TRANS-4-AMINOMETHYLCYCLOHEXANE-1-CARBOXYLIC ACID | C8 H15 N 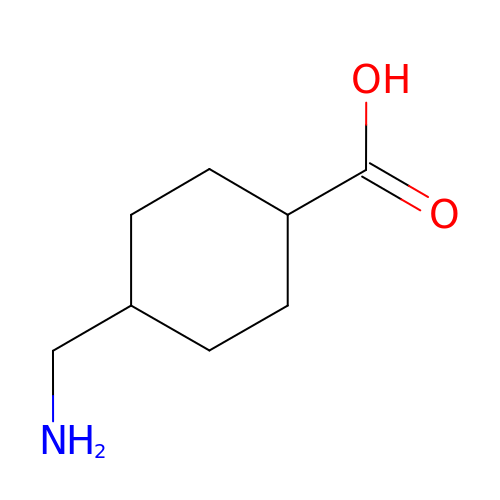O2 | GYDJEQRTZSCIOI-LJGSYFOKSA-N>[4x]MSQSVSERTRIKSDRYESGVIPYAKMGYWDASYTVKDTDVLALFRITPQPGVDPVEAAAAVAGESSTATWTVVWTDLLTACERYRAKAYRVDPVPNSADVFFAFIAYECDLFEEASLANLTASIIGNVFGFKAVSALRLEDMRIPHSYLXTFQGPATGIIVERERLNKYGTPLLGATVKPKLGLSGKNYGRVVYEGLKGGLDFLKDDENINSQPFMRWRERFLNCMEGINRASAATGEVKGSYLNITAATMEEVYKRAEYAKAVGSIVVMIDLVMGYTAIQSIAYWARENDMLLHLHRAGNSTYARQKNHGIN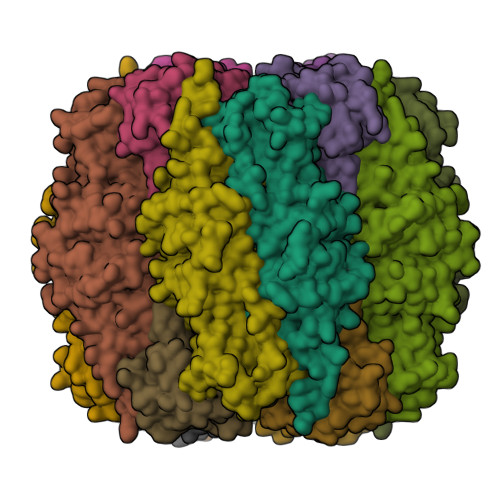FRVICKWMRMSGVDHIHAGTVVGKLEGDPLMIKGFYDILRLTELEVNLPFGIFFEMDWASLRRCMPVASGGIHCGQMHQLIHYLGDDVVLQFGGGTIGHPDGIQAGATANRVALESMVLARNEGVDYFDQQVGPQILRDAAKTCGPLQTALDLWKDISFDYTSTDTADFAE;>MRLTQGCFSFLPDLTDAQIEKQVAYAMAKGWAMNVEWTDDPHPRNNYWELWGLPLFDIKDPATVMFELNEARKSCAAGYIRINAFDASYGVESCVMSFITNRPTNEPGFYLDRTDGPGRQIVYSIKSYSVQANPEGSRY[4x]pmcA Disintegrin and Metalloproteinase 8 (ADAM8) is a transmembrane protein belonging to the metzincin superfamily of metalloproteases. ADAM8 is activated by autocatalysis in the trans-Golgi network and, for in vivo activity, requires the homophilic multimerization of at least two ADAM8 monomers on the cell membrane. In this context, the binding of a bifunctional ligand to the catalytic sites of an ADAM8 active homodimer on the tumor cell membrane could efficiently reduce ADAM8-mediated tumor growth and invasion to the surrounding tissues. In particular, we chose to dimerize the arylsulfonamido-based hydroxamic acid JG26,14 which has already been reported as a nanomolar ADAM17 inhibitor with a good selectivity over MMPs and ADAM10.

Considering the good fitting in ADAM8, JG26 was dimerized in the P1 position through the insertion of a N,N′-bis(carbamoyl-propyl)-isophthalamide spacer to give compound 1. X-ray crystallographic analysis in MMP-12 cd taken as model metalloprotease and molecular modeling studies in ADAM8 cd validated the design of 1, driving the synthesis of two other analogues bearing linkers of different lengths. Crystallographic analysis showed that the crystal of MMP-12 in complex with compound 1 belongs to space group C2 (cell parameters a = 51.291, b = 60.39, c = 54.00; β = 115.23°). The bifunctional inhibitor 1 (assigned occupancy 0.5) crosses the crystallographic two-fold axis of the MMP-12 homodimer, generating a trimeric adduct: MMP-12–1–MMP-12. In detail, the two hydroxamic acid groups of compound 1 chelate the two zinc ions of the MMP-12 homodimer, thus orienting the 3,5-dibromobiphenyl groups into the S1′ cavities. To verify if this arrangement could also be plausible for the ADAM8–1–ADAM8 trimer, we aligned two ADAM8–JG26 complexes on the MMP-12–1–MMP-12 adduct, maintaining the same N,N′-bis(carbamoyl-propyl)-isophthalamide spacer present in 1. The obtained complex was then subjected to 1.051 ms of MD simulation to analyze the stability of the trimeric complex. After ∼500 ns of MD simulation, the system reached a good stability, with the α-carbons of the two proteins showing an rmsd of ∼3.5 Å and the heavy atoms of compound 1 with an rmsd of ∼5.0 Å, thus confirming a good match between the experimental MMP-12–1–MMP-12 and the theoretical ADAM8–1–ADAM8 3D disposition.

> MGPVWRKHYITYRINNYTPDMNREDVDYAIRKAFQVWSNVTPLKFSKINTGMADILVVFARGAHGDDHAFDGKGGILAHAFGPGSGIGGDAHFDEDEFWTTHSGGTNLFLTAVHEIGHSLGLGHSSDPKAVMFPTYKYVDINTFRLSADDIRGIQSLYG> EVADFELMGVDGKTYRLSDYKGKKVYLKFWASWCSICLASLPDTDEIAKEAGDDYVVLTVVSPGHKGEQSEADFKNWY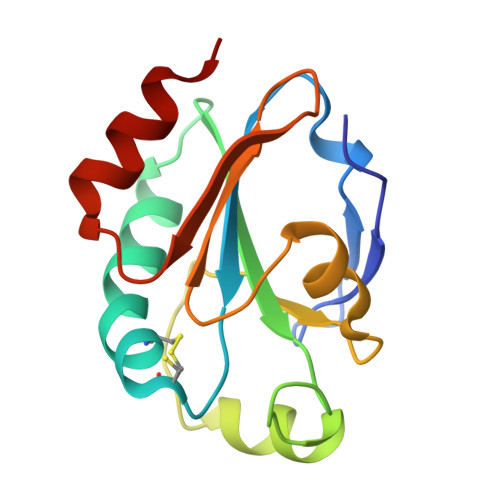KGLDYKNLPVLVDPSGKLLETYGVRSYPTQAFIDKEGKLVKTHPGFMEKDAILQTLKELA>[2x]MGHHHHHHGTQFEVLKQQKEIIEQGIDLFNKKPKRGIQYLQEQGMLGTTPEDIAQFLHQEERLDSTQVGEFLGDNDKFNKEVMYAYVDQHDFSGKDFVSALRMFLEGFRL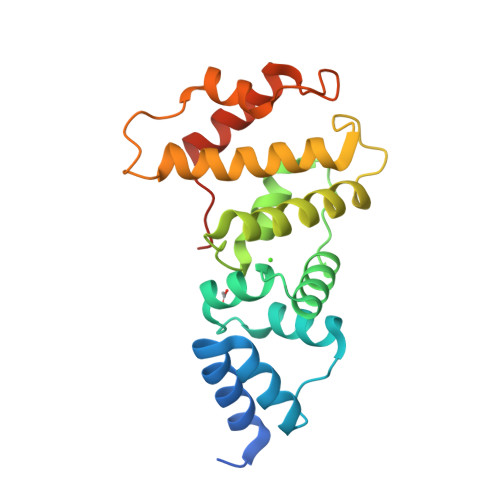PGEAQKIDRLMEKFAARYLECNQGQTLFASADTAYVLAYSIIMLTTDLHSPQVKNKMTKEQYIKMNRGINDSKDLPEEYLSAIYNEIAGKKISMKETKETG>[12x]MMNNKVSFTNSNNPTISLSAVIYFPPKFDETRQYQAIVLSHPGGGVKEQTAGTYAKKLAEKGFVTIAYDASYQGESGGEPRQLENPYIRTEDISAVIDYLTTLSYVDNTRIGAMGICAGAGYTANAAIQDRRIKAIGTVSAVNIGSIFRNGWENNVKSIDALPYVEAGSNARTSDISSGEYAIMPLAPMKESDAPNEELRQAWEYY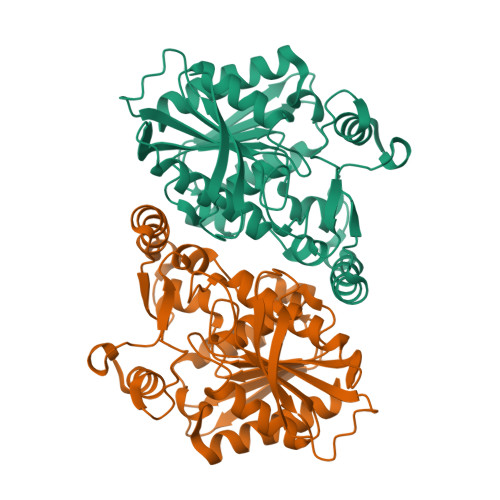HTPRAQYPTAPGYATLRSLNQIITYDAYHMAEVYLTQPTQIVAGSQAGSKWMSDDLYDRASSQDKRYHIVEGANHMDLYDGKAYVAEAISVLAPFFEETL> MKIREIIPLLSSNPLFSKTPQSSQKPSSFTSENNELSFTAKNFLSVNNQSSEIYYYSPIECKLYVIKVESTLDNTICAIRFQELKLKINFEVYKIELNEDSRYLCISGHVNCIIVDLNPQTVNSYFTSQEIFSDQENKTFGYDSLTVRSFTLDKTFYQSQISNIIKQVEWHPLSNIHLVILYSNNTLKIYNIQSGNEEIEQTFNLESIHTFESLKNLKNNDIRNQTKNTKKFISFCFGSNINFWTRFTIFLLSDSGEIFNLCPVIPNNCLVETSFYRDFQNHILYEKNQIENNSGSGSSNGDDSDEFIKQQQQQKKYYDFQFKWLMAASINTIPFEIENVSWLKLSSPSNSSTTFNPLLQGPISRISDSLPPSSNRVPLKILSIQPLVSNIDQNSNSSIINKINNNNNNDDDDNNNNNNNNNNNNNNNNNNDNDNDDDEKKKHNLSLSSTNKLIPFVIIVLMESCESLVNICCQDTIPMWSNDNGILYLEENNSNSNSKKQQQQQQQQQQPKYIDLILYEILDLNVKKSIKPSFSNIDKNLKN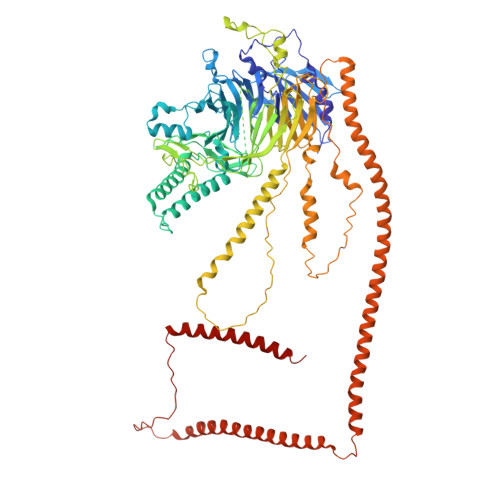KSTIAIASTNQTKDYLSYSLPTMKYDQWSDSLYFYHNQGVQIAKFPWLYQIYLEINNIVAFENNNNNNNNNNNNNKNNINNSSTTNNNNNKNKNKNDEIDENIEFETTSLMSVINNGSGNGDQCIPIIGIQVFSNIKIGTYFLILPNTFKIIIFDMDGLINQQPNLHEQKQQQQQNDDNDDDDDDDDNDEDEINLKSPIQPFIDNPPSFIGRIILPNSFTQKEFLQTLVNTKKKLYNLYIYSNQLEIELNSRVKGLELISKDQLKLIDKLKIYIENLKSNQQALNAKLKYVWDKKEIDSEEIKELYKVEMEGKPLSNQEKELAKTLKQINSQVNIYSERLNQVEKDLQENNNNNNNNNNNNSSNINNNNNNNGLISVTSYETIPIEHQTEIKKVLNLHGQKIEEDVTKLEKLLKNIQI>MWSHPQFEKASGTFYDVIEDYRHFDFAAYFAKVTDSDVRRILRQDRLSALDFLTLLSPQAEAYLEEMAQKAHRLTVQHFGRTMLLYTPLYLANYCVNQCVYCGFQLKNKLERKKLTLAEVEQEAQLIAATGLKHILILTGESRQHSPVSYIKDCVNILKKYFSSISIEIYPLTQEEYAELIGAGVDGLTIYQEVYNEEVYAEMHPAGPKRNYRFRLEAPERACQAGMRTVNIGALLGLNDWRQEAFFTGLHADYLQRRFPDVEVSISPPRMRPHLGGFPPRVVVSDQNLVQYVLAFRLFMPRSGITLSTRENGRLRDAMVRLGVTKMSAGSCTAVGGRSDQEAV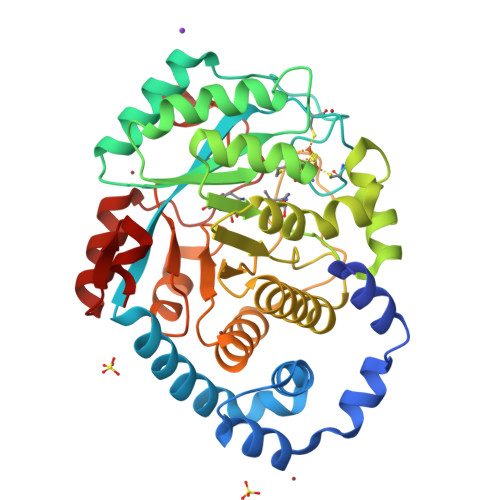GQFQISDERTVAEVAAMLYAQGYQPVYKDWQAL[2x]> MISKDEILEIFDKYNKDEITIATLGSHTSLHILKGAKLEGFSTVCITMKGRDVPY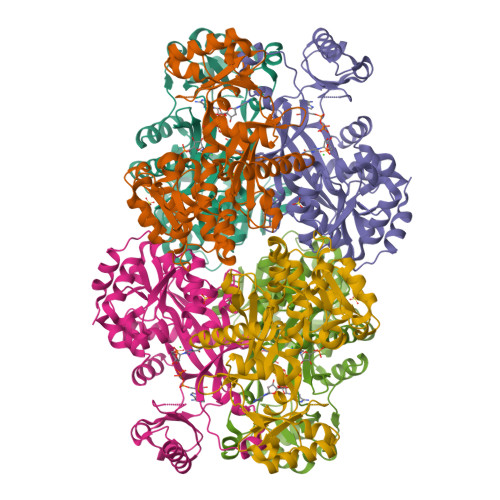KRFKVADKFIYVDNFSDIKNEEIQEKLRELNSIVVPHGSFIAYCGLDNVENSFLVPMFGNRRILRWESERSLEGKLLREAGLRVPKKYESPEDIDGTVIVKFPGARGGRGYFIASSTEEFYKKAEDLKKRGILTDEDIANAHIEEYVVGTNFCIHYFYSPLKDEVELLGMDKRYESNIDGLVRIPAKDQLEMNINPSYVITGNIPVVIRESLLPQVFEMGDKLVAKAKELVPPGMIGPFCLQSLCNENLELVVFEMSARVDGGTNSFMNGGPYSFLYNGEPLSMGQRIAREIKMALQLDMIDKIIS>GSAVMDHVSDSFLETNVPLLVLIEAAKNGNEKEVKEYAQVFREHANKLIEVANLACSISNNEEGVKLVRMSASQLEALCPQVINAALALAAKPQSKLAQENMDLFKEQWEKQVRVLTDAVDDITSIDD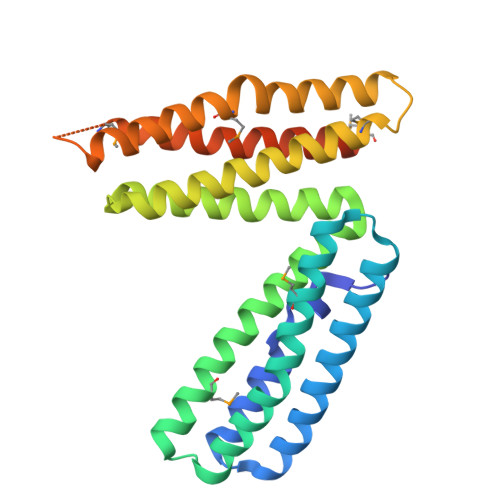FLAVSENHILEDVNKCVIALQEKDVDGLDRTAGAIRGRAARVIHVVTSEMDNYEPGVYTEKVLEATKLLSNTVMPRFTEQVEAAVEALSSDPAQPMDENEFIDASRLVYDGIRDIRKAVLMIRTPEELDDSDFETEDFDVR[3x]> GLTPEQKQKKAALSASEGEEVPQDKAPSHVPFLLIGGGTAAFAAARSIRARDPGARVLIVSEDPELPYMRPPLSKELWF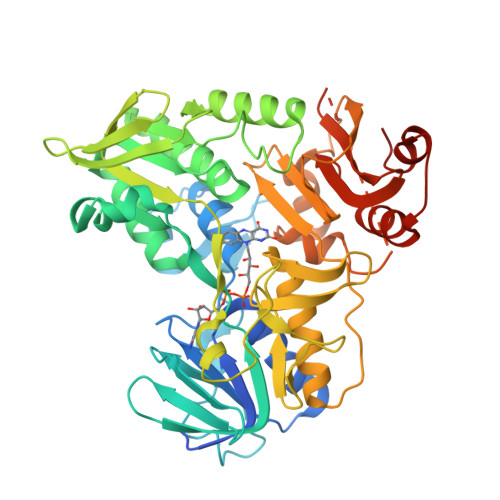SDDPNVTKTLRFKQWNGKERSIYFQPPSFYVSAQDLPHIENGGVAVLTGKKVVQLDVRDNMVKLNDGSQITYEKCLIATGGTPRSLSAIDRAGAEVKSRTTLFRKIGDFRSLEKISREVKSITIIGGGFLGSELACALGRKARALGTEVIQLFPEKGNMGKILPEYLSNWTMEKVRREGVKVMPNAIVQSVGVSSGKLLIKLKDGRKVETDHIVAAVGLEPNVELAKTGGLEIDSDFGGFRVNAELQARSNIWVAGDAACFYDIKLGRRRVEHHDHAVVSGRLAGENMTGAAKPYWHQSMFWSDLGPDVGYVAIGLVDSSLPTVGVFAKATAQDNPKSATEQSGTGIRSESETESEASEITIPPSTPAVPQAPVQGEDYGKGVIFYLRDKVVVGIVLWNIFNRMPIARKIIKDGEQHEDLNEVAKLFNIHEDLVP>[2x]MTCDDLKSGEKRLIPKPTCRFKDAFQQYPDLLKSIIRVGILKPTPIQSQAWPIILQGIDLIVVAQTGTG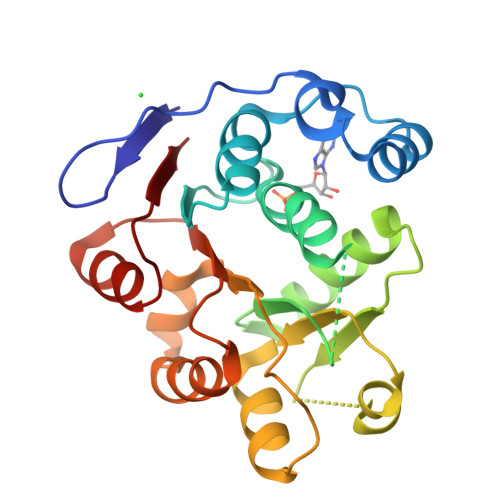KTLSYLMPGFIHLDSQPISREQRNGPGMLVLTPTRELALHVEAECSKYSYKGLKSICIYGGRNRNGQIEDISKGVDIIIATPGRLNDLQMNNSVNLRSITYLVIDEADKMLDMEFEPQIRKILLDVRPDRQTVMTSATWPDTVRQLALSYLKDPMIVYV> APDWVPPEVFDLVAEDKARCMSEHGTTQAQIDDVNKGNLVNEPSITCYMYCLLEAFSLVDDEANVDEDIMLGLLPDQLQERAQSVMGKCLPTSGSDNCNK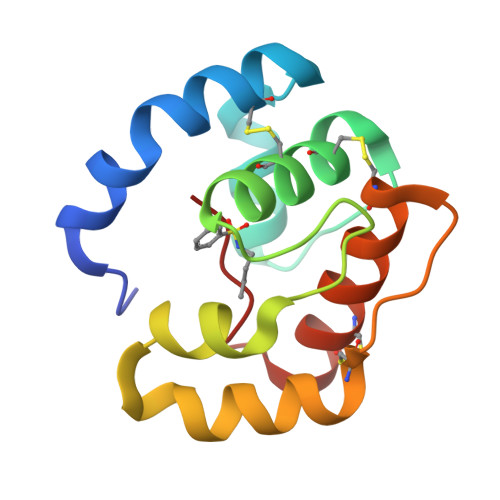IYNLAKCVQESAPDVWFVI1-({[(S)-hydroxy(phosphonooxy)phosphoryl]oxy}acetyl)-L-proline | C7 H13 N O10 P2 | 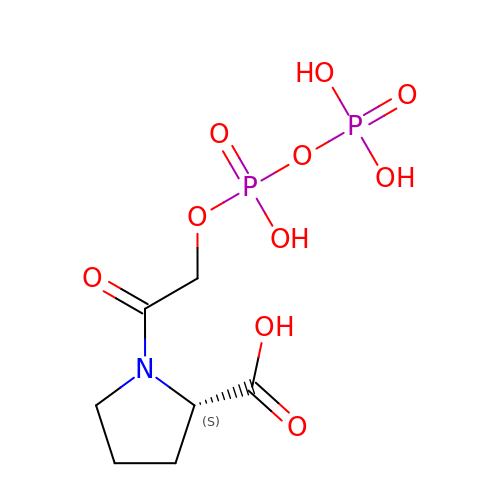JFTJDUMMWOSHFL-YFKPBYRVSA-N>[4x]AKKIILDCDPGLDDAVAILLAHGNPEIELLAITTVVGNQTLAKVTRNAQLVADIAGITGVPIAAGCDKPLVRKIMTAGHIHGESGMGTVAYPAEFKNKVDERHAVNLIIDLVMSHEPKTITLV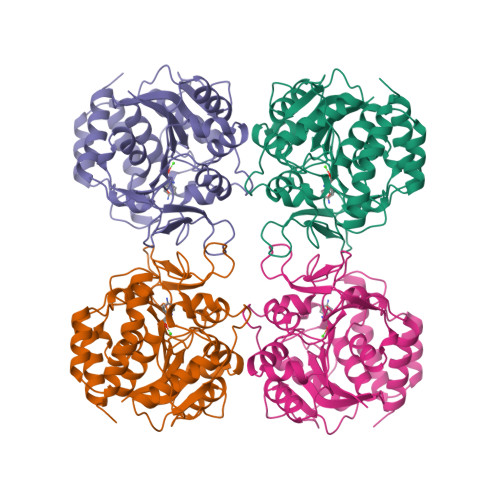PTGGLTNIAMAARLEPRIVDRVKEVVLMGGGYHEGNATSVAEFNIIIDPEAAHIVFNESWQVTMVGLDLTHQALATPPILQRVKEVDTNPARFMLEIMDYYTKIYQSNRYMAAAAVHDPCAVAYVIDPSVMTTERVPVDIELTGKLTLGMTVADFRNPRPEHCHTQVAVKLDFEKFWGLVLDALERIGDPQ>MAGNREDRKAKVIEVLNKARAMELHA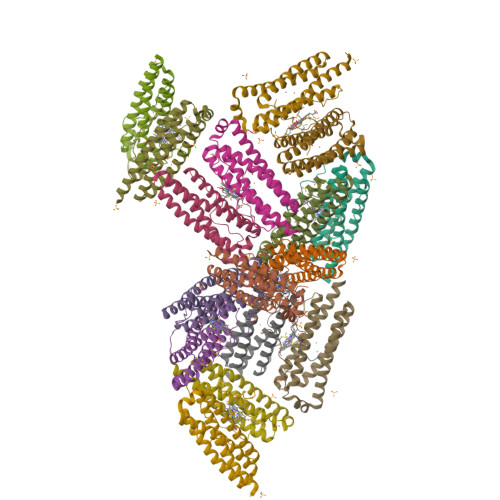IHQYMNQHYSLDDMDYGELAANMKLIAIDEMRHAENFAERIKELGGEPTTQKEGKVVTGQAVPVIYESDADQEDATIEAYSQFLKVCKEQGDIVTARLFERIIEEEQAHLTYYENIGSHIKNLGDTYLAKIAGTPSSTGTASKGFVTATPAAE[16x]>MDEALIKDYHSIREQIDQYTKDMVLVMQHPTNCVKYINPGRLMHVVTSDGTDFGWGVIINFYERRPERNNPNPGWSPQESYVVEVLLRLSSDSGSVDSKLKDNQCIPAGIAPVTQKNDPGRWEVVPCLLSCMHGLSQIKLHVPDKKSGGSMDDPETRRRVGKSLLEVQRRFEDGIPHMDPIENMHIRDVEFKKLLRKIEVLESRLVANPLHNSGGSGGS[2x];>[2x]ALSYSSPLRFFRNFRFHPEFTRLVAGGWRSLTYSSRIDPDKEMCPYELEGTQC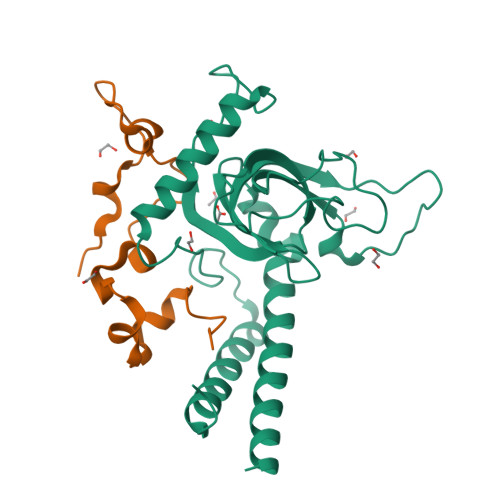PSGCSFQHFVDITPAADERILLELSGSHHHHHH>[2x]TRDQNGTWEMESNENFEGYMKALDIDFATRKIAVRLTQTLVIDQDGDNFKVKTTSTFRNYDVDFTVGVEFDEYTKSLDNRHVKALVTWEGDV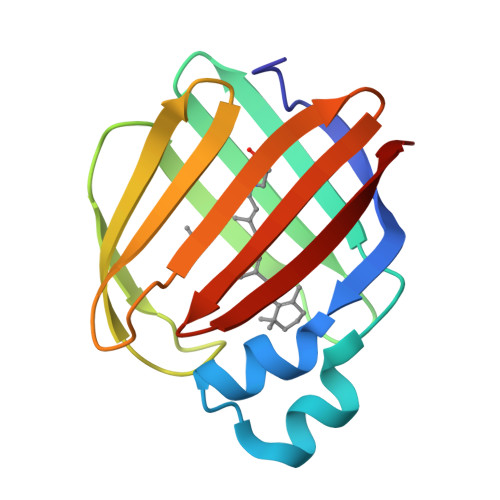LVCVQKGEKENRGWKKWIEGDKLYLELTCGDQVCRQVFKKK> QTIRSASDIRDVFINAGIKGEEYDAAWNSFVVKSLVAQQEKAAADVQLRGVPAMFVNGKYQLNPQGMDTSNMDVFVQQYADTVKYLSEKKGGGTGAQYEDGKQYTTLEKPVAGAPQVLEFFSFFCPHCYQFEEVLHISDNVKKKLPEGVKMTKYHVNFMGGDLGKD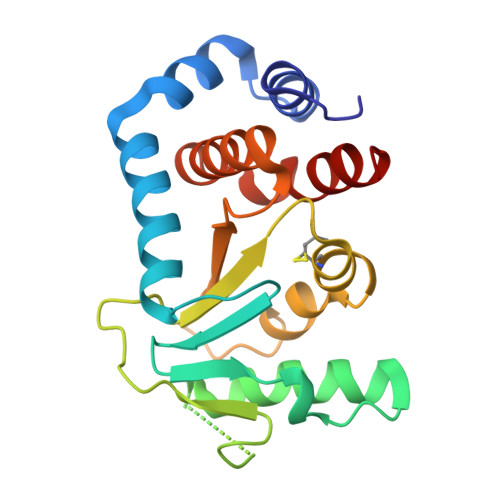LTQAWAVAMALGVEDKVTVPLFEGVQKTLIK> MTSLIDLGRYVERTHHGEDTEPRSKRVKIAKPDLSSFQPGSIIKIRLQDFVTYTLTEFNLSPSLNMIIGPNGSGKSTFVCAVCLGLAGKPEYIGRSKKVEDFIKNGQDVSKIEITLKNSPNVTDIEYIDARDETIKITRIITRSKRRSDYLINDYQVSESVVKTLVAQLNIQLDNLCQFLSQERVEEFARLKSVKLLVETIRSIDASLLDVLDELRELQGNEQSLQKDLDFKKAKIVHLRQESDKLRKSVESLRDFQNKKGEIELHSQLLPYVKVKDHKEKLNIYKEEYERAKANLRAILKDKKPFANT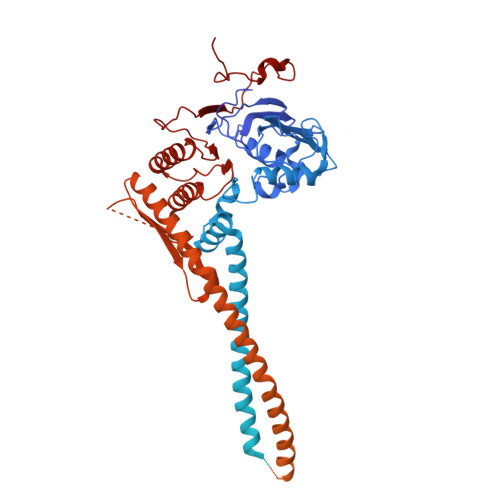KKTLENQVEELTEKCSLKTDEFLKAKEKINEIFEKLNTIRDEVIKKKNQNEYYRGRTKKLQATIISTKEDFLRSQEILAQTHLPEKSVFEDIDIKRKEIINKEGEIRDLISEIDAKANAINHEMRSIQRQAESKTKSLTTTDKIGILNQDQDLKEVRDAVLMVREHPEMKDKILEPPIMTVSAINAQFAAYLAQCVDYNTSKALTVVDSDSYKLFANPILDKFKVNLRELSSADTTPPVPAETVRDLGFEGYLSDFITGDKRVMKMLCQTSKIHTIPVSRRELTPAQIKKLITPRPNGKILFKRIIHGNRLVDIKQSAYGSKQVFPTDVSIKQTNFYQGSIMSNEQKIRIENEIINLKNEYNDRKSTLDALSNQKSGYRHELSELASKNDDINREAHQLNEIRKKYTMRKSTIETLREKLDQLKREARKDVSQKIKDIDDQIQQLLLKQRHLLSKMASSMKSLKNCQKELISTQILQFEAQNMDVSMNDVIGFFNEREADLKSQYEDKKKFVKEMRDTPEFQSWMREIRSYDQDTKEKLNKVAEKYEEEGNFNLSFVQDVLDKLESEIAMVNHDESAVTILDQVTAELRELEHTVPQQSKDLETIKAKLKEDHAVLEPKLDDIVSKISARFARLFNNVGSAGAVRLEKPKDYAEWKIEIMVKFRDNAPLKKLDSHTQSGGERAVSTVLYMIALQEFTSAPFRVVDQINQGMDSRNERIVHKAMVENACAENTSQYFLITPKLLTGLHYHEKMRIHCVMAGSWIPNPSEDPKMIHFGETSNYSFD> NPVENYIDEVLNEVLVVPNINSSNPTTSNSAPALDAAETGHTSSVQPEDVIETRYVQTSQTRDEMSLESFLGRSGCIHESKLEVTLANYNKENFTVWAINLQEMAQIRRKFELFTYTRFDSEITLVPCISALSQDIGHITMQYMYVPPGAPVPNSRDDYAWQSGTNASVFWQHGQAYPRFSLPFLSVASAYYMFYDGYDEQDQNYGTANTNNMGSLCSRIVTEKHIHKVHIMTRIYHKAKHVKAWCPRPPRALEYTRAHRTNFKIEDRSIQTAIVTRPIITTA;> SPTVEACGYSDRIIQITRGDSTITSQDVANAIVAYGVWPHYLSSKDASAIDKPSQPDTSSNRFYTLRSVTWSSSSKGWWWKLPDALKDMGIFGENMFYHYLGRSGYTIHVQCNASKFHQGTLIVALIPEHQIASALHGNVNVGYNYTHPGETGREVKAET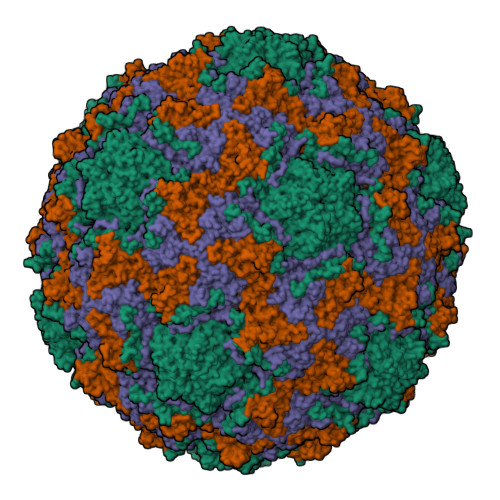RLNPDLQPTEEYWLNFDGTLLGNITIFPHQFINLRSNNSATIIAPYVNAVPMDSMRSHNNWSLVIIPICPLETSSAINTIPITISISPMCAEFSGARAKRQ;> GLPVFITPGSGQFLTTDDFQSPCALPWYHPTKEISIPGEVKNLVEICQVDSLVPINNTDTYINSENMYSVVLQSSINAPDKIFSIRTDVASQPLATTLIGEISSYFTHWTGSLRFSFMFCGTANTTVKLLLAYTPPGIAEPTTRKDAMLGTHVIWDVGLQSTISMVVPWISASHYRNTSPGRSTSGYITCWYQTRLVIPPQTPPTARLLCFVSGCKDFCLRMARDTNLHLQSGAIAQ;> GAQVSRQNVGTHSTQNSVSNGSSLNYFNINYFKDAASNGASKLEFTQDPSKFTDPVKDVLEKGIPTLQ> GAMGTRDDEYDYLFKVVLIGDSGVGKSNLLSRFTRNEFNLESKSTIGVEFATRSIQVDGKTIKAQIWDTAGQERYRAITSAYYRGAVGALLVYDIAKHLTYENVERWLKELRDHADSNIVIMLVGNKSDLRHLRAVPTDEARAFAEKN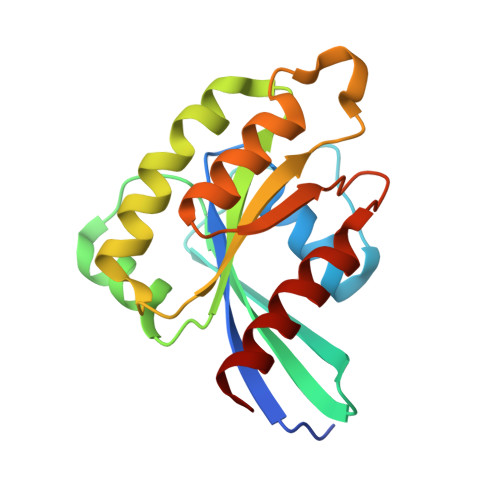GLSFIETSALDSTNVEAAFQTILTEIYRIVS9H-CARBAZOLE | C12 H9 N | 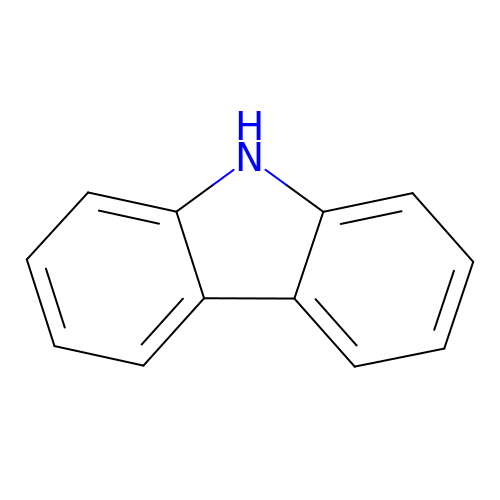UJOBWOGCFQCDNV-UHFFFAOYSA-N>GSSMDNQDGFILQQVKLSLDDPDSYLSSWNSNDASPCRWSGVSCAGDFSSVTSVDLSSANLAGPFPSVICRLSNLAHLSLYNNSINSTLPLNIAACKSLQTLDLSQNLLTGELPQTLADIPTLVHLDLTGNNFSGDIPASFGKFENLEVLSLVYNLLDGTIPPFLGNISTLKMLNLSYNPFSPSRIPPEFGNLTNLEVMWLTECHLVGQIPDSLGQLSKLVDLDLALNDLVGHIPPSLGGLTNVVQIELYNNSLTGEIPPELGNLKSLRLLDASMNQLTGKIPDELCRVPLESLNLYENNLEGELPASIALSPNLYEIRIFGNRLTGGLPKDLGLNSPLRWLDVSENEFSGDLPADLCAKGELEELLIIHNSFSGVIPESLADCRSLTRIRLAYNRFSGSVPTGFWGLPHVNLLELVNNSFSGEISKSIGGASNLSLLILSNNEFTGSLPEEIGSLDNLNQLSASGNKFSGSLPDSLMSLGELGTLDLHGNQFSGELTSGIKSWKKLNELNLADNEFTGKIPDEIGSLSVLNYLDLSGNMFSGKIPVSLQSLKLNQLNLSYNRLSGDLPPSLAKDMYKNSFIGNPGLCGDIKGLCGSENEAKKRGYVLEGSENLYFQ[2x];>GSSMASANLEGDALHTLRVTLVDPNNVLQSWDPTLVNPCTWFHVTCNNENSVIRVDLGNAELSGH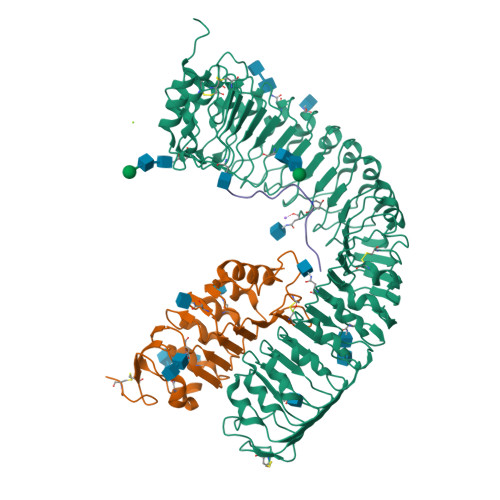LVPELGVLKNLQYLELYSNNITGPIPSNLGNLTNLVSLDLYLNSFSGPIPESLGKLSKLRFLRLNNNSLTGSIPMSLTNITTLQVLDLSNNRLSGSVPDNGSFSLFTPISFANNLDLCGPVTSHPCPLEGSLENLYFQ[2x];>YVPIPPSAPSKRHN[2x]> VPPALHLVDPQIQLTITDPKVYPIILRLGSNLSLSMARRNLDSLEARAFQSTPIVV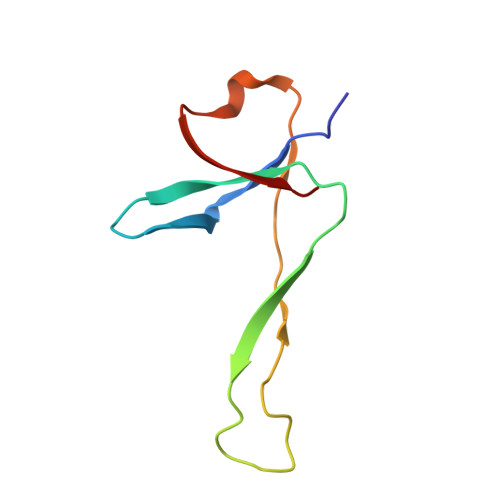QMTKLATTEELPDEFVVVTAK> YEYVELAKASLTSAQPQHFYAVVIDATFPYKTNQERYICSLKIVDPTLYLKQQKGAGDASDYATLVLYAKRFEDLPIIHRAGDIIRVHRATLRLYNGQRQFNANVFYSSSWALFSTDK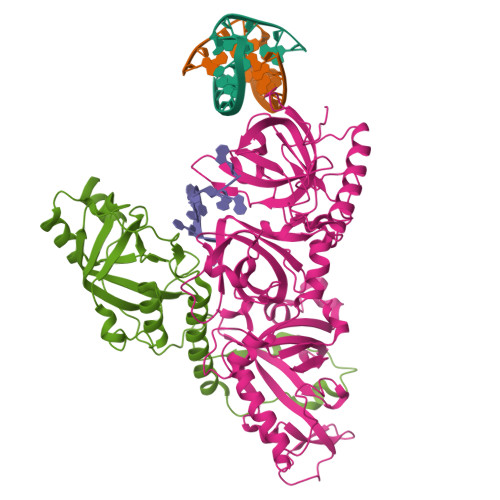RSVTQEINNQDAVSDTTPFSFSSKHATIEKNEISILQNLRKWANQYFSSYSVISSDMYTALNKAQAQKGDFDVVAKILQVHELDEYTNELKLKDASGQVFYTLSLKLKFPHVRTGEVVRIRSATYDETSTQKKVLILSHYSNIITFIQSSKLAKELRAKIQDDHSVEVASLKKNVSLNAVVLTEVDKKHAALPSTSLQDLFHHADSDKELQAQDTFRTQFYVTKIEPSDVKEWVKGYDRKTKKSSSLKGASGKGDNIFQVQFLVKDASTQLNNNTYRVLLYTQDGLGANFFNVKADNLHKNADARKKLEDSAELLTKFNSYVDAVVERRNGFYLIKDTKLI;> QQQSAFKQLYTELFNNEGDFSKVSSNLKKPLKCYVKESYPHFLVTDGYFFVAPYFTKEAVNEFHAKFPNVNIVDLTDKVIVINNWSLELRRVNSAEVFTSYANLEARLIVHSFKPNLQERLNPTRYPVNLFRDDEFKTTIQHFRHTALQAAINKTVKGDNLVDISKVADAAGKKGKVDAGIVKASASKGDEFSDFSFKEGNTATLKIADIFVQEKG>GRKERERLEEKLEDANERIAELVKLEERQRIARDLEDTLGQKLSLIGLKSDLARKLIYKDPEQAARELKSVQQTARTSLNEVRKIVSSMKGIRLKDELINIKQILEAADIMFIYEEEKWPENISLLNENILSMCLKEAVTNVVKHSQAKTCRVDIQQLWKEVVITVSDDGTFKGEENSFSKGHGLLGMRERLEFANGSLHIDTENGTKLTMAIPNNSK[4x];>GSGSMISIFIAEDQQMLLGALGSLLNLEDDMEVVGKGTTGQDAVDFVKKRQPDVCIMDIEMPGKTGLEAAEELKDTGCKIIILTTFARPGYFQRAIKAGVKGYLLKDSPSEELANAIRSVMNGKRIYAPELMEDLYSEA[2x]

The simplest TCSs comprise a sensory histidine kinase (HK) and a response regulator (RR) component. To address this question we have used the TCS DesK-DesR from B. subtilis as a model. We had previously shown that the HK DesK, a member of the HisKA_3 family, undergoes important conformational changes to switch between phosphatase- and phosphotransfer-competent states. We now report the crystal structures of the DesKC:DesR complex, trapped in the phosphatase and the phosphotransferase functional states.

One using the phosphatase-constitutive mutant DesKCSTAB, and the other with DesKCH188E carrying a phosphomimetic substitution, both in complex with the REC domain of DesR. (D) Cartoon representation of the DesKCH188E:DesR-REC (phosphotransferase) complex, along two orthogonal views (left and right subpanels). Note best fitting with a one dimer DesKCH188E (chains AB) to one monomer DesR-REC (chain C) model. The structures show the RR REC domain adopting identical conformations in both phosphatase and phosphotransferase complexes, presenting active- and inactive–like features in different regions of the protein, arranging the RR’s active site for phosphoryl group migration. Except for the phosphate lid, the REC domain bound to the HK largely resembles the RR’s active form, shifting the position of the β1α1 loop and helix α1, now able to recruit the Mg2+ cation essential for phosphoryl-transfer catalysis. The β4α4 loop in DesR plays a key role in these controls, remodeling its configuration in concert with DesK-association. This loop, acting as a phosphate lid, is open in the phosphotransferase complex, enabling the transfer reaction. Binding to unphosphorylated RR positions the P~His188(HK) into a suitable orientation for phosphoryl-transfer to occur through a loose (dissociative) nucleophilic substitution. Taking into account that phosphotransfer is a nucleophilic substitution at phosphorus, the reaction coordinate distance (i.e. between phosphorus and the entering atom, before the transfer reaction has begun) strongly suggests that P~DesK→DesR phosphotransfer occurs through a largely dissociative, or ‘loose’ mechanism: a reaction coordinate distance of ≥4.9 Å provides room for a fully dissociated metaphosphate intermediate. The His-Asp distance thus correlates with associative vs dissociative phosphotransfer, but also with the symmetry of the Mg2+ cation with respect to the entering and leaving atoms. The phosphatase/phosphotransferase transition, switches the distance and orientation of the HK histidine side chain with respect to the RR aspartate, enabling for the distinct reaction mechanisms to take place, and ultimately ensuring the unidirectional flow of information.>[4x]MVKPNWDNFKAKFSENPQGNFEWFCYLLFCQEFKMPAGIFRYKNQSGIETNPITKDNEIIGWQSKFYDTKLSDNKADLIEMIEKSKKAYPGLSKIIFYTNQEWGQGRKSHEPEGDKNADNYLETVGNSNDPKIKIEVDQKAYESGIEIVWRVASFFESPFVIVENEKIAKHFFSLNESIFDLLEEKRKHTENVLYEIQTNIEFKDRSIEIDRRHCIELLHENLVQKKIVIVSGEGGVGKTAVIKKIYEAEKQYTPFYVFKASEFKKDSINELFGAHGLDDFSNAHQDELRKVIVVDSAEKLLELTNIDPFKEFLTVLIKDKWQVVFTTRNNYLADLNYAFIDIYKITPGNLVIKNLERGELIELSDNNGFSLPQDVRLLELIKNPFYLSEYLRFYTGESIDYVSFKEK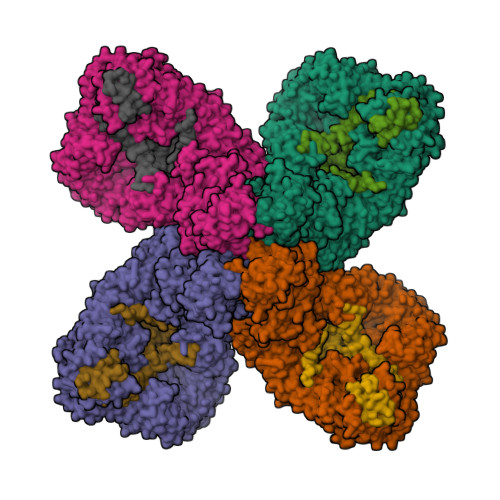LWNKIIVKNKPSREQCFLATAFQRASEGQFFVSPACDTGILDELVKDGIVGYEAAGYFITHDIYEEWALEKKISVDYIRKANNNEFFEKIGESLPVRRSFRNWISERLLLDDQSIKPFIAEIVCGEGISNFWKDELWVAVLLSDNSSIFFNYFKRYLLSSDQNLLKRLTFLLRLACKDVDYDLLKQLGVSNSDLLSIKYVLTKPKGTGWQSVIQFIYENLDEIGIRNINFILPVIQEWNQRNKVGETTRLSSLIALKYYQWTIDEDVYLSGRDNEKNILHTILHGAAMIKPEMEEVLVKVLKNRWKEHGTPYFDLMTLILTDLDSYPVWASLPEYVLQLADLFWYRPLKETGERYHSMDIEDEFGLFRSHHDYYPESPYQTPIYWLLQSQFKKTIDFILDFTNKTTICFAHSHFAKNEIEEVDVFIEEGKFIKQYICNRLWCSYRGTQVSTYLLSSIHMALEKFFLENFKNADSKVLESWLLFLLRNTKSASISAVVTSIVLAFPEKTFNVAKVLFQTKDFFRFDMNRMVLDRTHKSSLISLRDGFGGTDYRNSLHEEDRIKACDDVHRNTYLENLALHYQIFRSENVTEKDAIERQQVLWDIFDKYYNQLPDEAQETEADKTWRLCLARMDRRKMKITTKEKDEGIEISFNPEIDPKLKQYSEEAIKKNSEHMKYVTLKLWASYKREKDERYKNYGMYEDNPQIALQETKEIIKKLNEEGGEDFRLLNGNIPADVCSVLLLDYFNQLNNEEREYCKDIVLAYSKLPLKEGYNYQVQDGTTSAISALPVIYHNYPMERETIKTILLLTLFNDHSIGMAGGRYSVFPSMVIHKLWLDYFDDMQSLLFGFLILKPKYVILSRKIIHESYRQVDYDIKKININKVFLNNYKHCISNVIDNKISIDDLGSMDKVDLHILNTAFQLIPVDTVNIEHKKLVSLIVKRFSTSLLSSVREDRVDYALRQSFLERFAYFTLHAPVSDIPDYIKPFLDGFNGSEPISELFKKFILVEDRLNTYAKFWKVWDLFFDKVVTLCKDGDRYWYVDKIIKSYLFAESPWKENSNGWHTFKDSNSQFFCDVSRTMGHCPSTLYSLAKSLNNIASCYLNQGITWLSEILSVNKKLWEKKLENDTVYYLECLVRRYINNERERIRRTKQLKQEVLVILDFLVEKGSVVGYMSRENIL;>MASSQKREGFAENGAKAVYDALKNDRNSYETRAENCAKYTIPSLFPKDSDNASTDYTTPWQAVGARGLNNLASKLMLALFPMQTWMKLTISEFEAKQLVAQPAELAKVEEGLSMVERILMNYIESNSYRVTLFETLKQLVVAGNALLYIPEPEGAYNPMKLYRLSSYVVQRDAFGTVLQIVTLDKTAYAALPEDVRNAMDSGQEHKGDEMIDVYTHIYLDEESGEYLKYEEIDGVEVDGTDASYPVDACPYIPVRMVRIDGESYGRSYCEEYLGDLRSLENLQEAIVKMSMISAKVIGLVNPAGITQVRRLTKAQTGDFVSGRPEDISFLQLEKAADFSVAKAVSEQIEGRLSYAFMLNSAVQRTGERVTAEEIRYVASELEDTLGGVYSILSQELQLPMVRVLLKQLQATNQIPELPKEAVEPTISTGMEALGRGQDLDKLERCIAAWSALAPMQNDPDINIATIKLRIANAIGIDTSGILKTPEEKQQEMAEAAQGTALENAAASAGAGAGALATASPENMEAAAAQAGMVPN[4x]Mutations in dysferlin, the first protein linked with the cell membrane repair mechanism, causes a group of muscular dystrophies called dysferlinopathies. Dysferlin, a member of the ferlin protein family, is a type II anchored membrane protein with a single C terminal helix buried in the membrane. Dysferlin is not a part of the dystrophin-glycoprotein complex, but its function is linked with calcium-activated membrane repair caused by fusing aggregated intracellular vesicles with the sarcolemma at the site of injury. One DysF domain is inserted into the other DysF domain, by gene duplication, forming an inner DysF domain and a two part (N terminal and C terminal) outer DysF domain.

In this study, we have determined the three dimensional structure of human dysferlin inner DysF domain by X-ray crystallography at 1.9 Å. The structure was solved by molecular replacement with the NMR structure of the inner DysF of myoferlin. Most datasets that were collected, processed and refined in space group P213 (cubic), with the best resolution dataset diffracting to 1.9 Å. Except where stated otherwise the analysis is based on the single chain in the 1.9 Å structure. The inner DysF domain construct starts at residue Met942 and ends at Gln1052 and has a Ser on the N terminus from the TEV protease site. The main secondary structure consists of two long antiparallel β-strands, one at each terminus (N terminus 946-958, C terminus 1036-1049). These β-strands are connected with a long loop (77 residues). As reported for the myoferlin inner DysF domain, the dysferlin DysF domain is held together by arginine/aromatic sidechain stacking. The analysis shows that in fact there is not one continuous stack, but three on one face of the sheet. The three most frequent mutations disrupt the R/W stacks and are likely to lead to a less stable or possibly unfolded domain.

> SMDAGHLSFVEEVFENQTRLPGGQWIYMSDNYTDVNGEKVLPKDDIECPLGWKWEDEEWSTDLNRAVDEQGWEYSITIPPERKPKHWVPAEKMYYTHRRRRWVRLRRRDLSQ>MKGPNLNFRKTPSKDNGVKQVESLARPETPPPKFVEDSNLEFNVLASEKLPNYTNLDLFHRAVFPFMFLAQCVAIMPLVGIRESNPRRVRFAYKSIPMFVTLIFMIATSILFLSMFTHLLKIGITAKNFVGLVFFGCVLSAYVVFIRLAKKWPAVVRIWTRTEIPFTKPPYEIPKRNLSRRVQLAALAIIGLSLGEHALYQVSAILSYTRRIQMCANITTVPSFNNYMQTNYDYVFQLLPYSPIIAVLILLINGACTFVWNYMDLFIMMISKGLSYRFEQITTRIRKLEHEEVCESVFIQIREHYVKMCELLEFVDSAMSSLILLSCVNNLYFVCYQLLNVFNKLRWPINYIYFWYSLLYLIGRTAFVFLTAADINEESKRGLGVLRRVSSRSWCVEVERLIFQMTTQTVALSGKKFYFLTRRLLFGMAGTIVTYELVLLQFDEPNRRKGLQPLCALEGGSSGGWSHPQFEK[4x]

While mammals use G protein-coupled receptors (GPCRs) for sweet and bitter tastant perception, insects such as fruit flies use a unique family of proteins called gustatory receptors (Grs). To unravel the overall structure of these receptors and their unique structure features that define sugar specificity, we determined the cryo-electron microscopy (cryo-EM) structures of Drosophila mojavensis Gr43a (DmoGr43a) (given its better biochemical behavior than Drosophila melanogaster Gr43a (DmGr43a)) and Drosophila melanogaster Gr64a (DmGr64a) in apo or sugar-bound states. As expected, both DmoGr43a and DmGr64a form tetramer, and are topologically similar to each other, and to Orco from Apocrypta bakeri and odorant receptor 5 from Machilis hrabei (MhOR5)11. The structures of DmoGr43a and DmGr64a can be separated into a TMD with 28 transmembranes (TMs) in total (7 TMs in each subunit, numbered as S1–S7), and an intracellular domain (ICD) containing an “anchor domain”, following the nomenclature of Orco/MhOR510,11.

For DmGr64a, among tested sugars, several sugars including fructose, trehalose, sucrose and maltose were able to activate DmGr64a in our calcium imaging experiments, whereas glucose and arabinose could not. Structure of DmGr64a is more expanded than that of DmoGr43a, particularly in the transmembrane domain (TMD), which appears to partially account for the differences in their sugar specificity. The sugar binding pocket is surrounded by S1–S6 in the TMD of each subunit in both proteins, with the one for DmGr64a being much larger, consistent with a wider sugar spectrum observed in DmGr64a. Larger sugar binding pocket in DmGr64a results from splaying of extracellular half of the helical bundle (S1–S6) that harbors the binding site. Among these helices, the extracellular halves of S1, S3, and S4 undergo the most dramatic outward tilting in DmGr64a when compared with DmoGr43a. Lined by S7 that spans both ICD (S7a) and TMD (S7b), a continuous ion conduction pathway in the 4-fold symmetry axis runs all the way through both DmoGr43a and DmGr64a, and are all in the non-conductive state. In both proteins, two patches of constrictions are formed along the ion conduction pathway, one near the extracellular entrance (Ile 418 and Phe 422 for DmoGr43a, and Val 438 and Gln 441 for DmGr64a) and the other in the anchor domain in ICD (Leu 386 for DmoGr43a, and Glu 399 and Phe 403 for DmGr64a). Intriguingly, the narrowest point at the extracellular entrance is formed by completely different sets of residues in DmoGr43a and DmGr64a, e.g., bulky, hydrophobic phenylalanine in DmoGr43a vs smaller, hydrophilic glutamine in DmGr64a. When the apo and sugar-bound structures of DmoGr43a and DmGr64a were aligned, notable conformational changes could be revealed, mainly tilting of TM helices responsible for sugar binding towards bound sugars.>GKSEISELRRTMQNLEIELQSQLSMKASLENSLEETKGRYAMQLAQIQEMIGSVEEQLAQLRCEMEQQNQEYKILLDVKTRLEQEIATYRRLLEG[2x];>[2x]LRNTKHEISEMNRMIQRLRAEIDNVKKQCANLQNAIADAEQRGELALKDARNKLAELEEALQKAKQDMARLLREYQELMNTKLALDVEIATY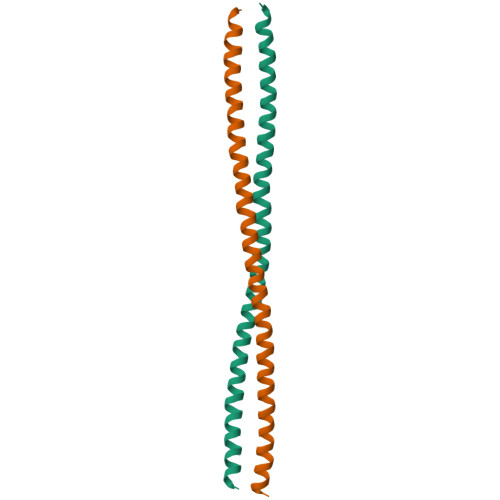RKLLEG>MRALIVYTELTDKDSVISHAVARLASELNDEHVETVIIRDFEDGLAYIRSNTSIDCLLYGRDMSDRDEQIQAHRLITQLHRRQEDVPVFLLS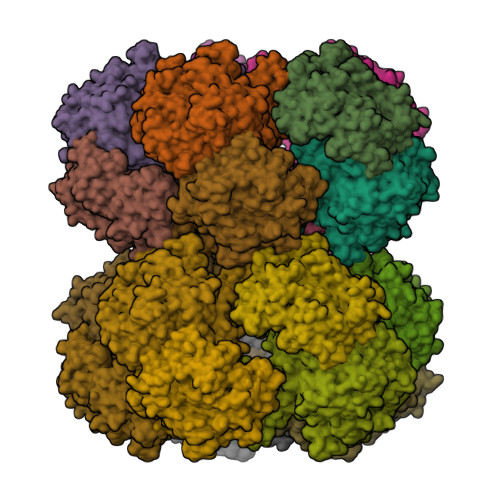DREEALVAFDRNMMEQVDEFAWILEDSADFIAGRVLAAIQRYRSQLLPPLMKSLIKYSDVHEYSWAAPGHQGGVGFTKTPAGRIYHDFFGENLFRTDIGIERVAVGSLLDHTGAFGECEKNAARIFGADQSYSVVVGTSGSNRTIMQACMTDDDVVVIDRNCHKSIEQGLILTGAKPVYMIPSRNRYGIIGPIYPKEMTPDAIKFKIAANPLTKGKVKQKPAYSVVTNCTYDGVCYNARKVQDLLDGSLDRIHFDEAWYGYARFNPLYRNHFAMRDEERTENEPTIFATHSTHKLLNALSQASFIHVRNGRNAIDFNRFNQAYLMHSTTSPLYAICASNDIAADMMDGNSGRSLTDEVIRESIDFRQSLAYLYKEFLNDDEWFFKPWNQEMVKDPATGKRYAFEDAPVELLMREQSCWVMHPEDKWHGFNDIPDNWAMLDPIKVSILAPGMGDDGKLLDTGVPAALVTAWLNHYGIVPTRTTDFQIMFLFSMGITKGKWGTLVNTLLSFKRHYDNNTALKKVLPEVVASAPEIYGEMGLRDLGDKMFAYLQKNNPGARLNQAYSQLPQVMMTPRDAYQQIVANRVEAVPVDQLMGRVAANSIIPYPPGIPMLLSGENFGDENSPHIHYLRSLQAWDSEFPGFEHETEGTEIIDGQYYVMCVKTCDE[20x]> MAITSVDSYLLSEIKPRLNTVLENCYIIDEVLKDFDYQTRESFKEAFCGKNAQHEVTVGFNFPKFKNNYEAHYLIQLGQGQET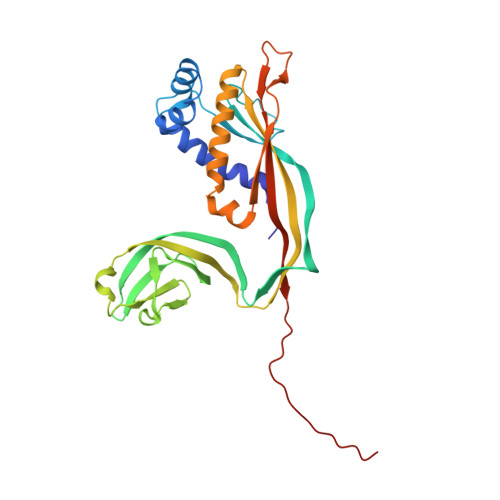KNSLGSIQSSYFEATGDTLVESSTAIREDDKLVFTVSKPIGELIKVEDIEFAKYDNLQVEGNKVSFKYQTNEDYENYNANIIFTEKKNDSKGLVKGFTVEEQVTVVGLSFNVDVARCLDAVLKMILISMRDSIEEQQTFQLQNLSFGDIAPIIEDGDSMIFGRPTIIKYTSSLDLDYTITQDINKLTFKERKDWK>GSAKDPVASAQIELIKQRINNIELFQNNRQAADSALRLEEGILSNAVNSLHRLREIQIQAGNPSLSEEDRKTLAVEAQALLNQLLDYANTKDSNGSYMFSGSKSLTQPVSLNLSGQYVYNGDSTQRFQAVTTSLLVAVNDTGDNVFMRIPSGNGRFAIRETLTPNTGTASVSSGSVTNEAAFVPDNYTMTFALNSQGNLVVMVSGTLSGNVIPPSGLPDDAPLYQEGSAIGFNGMEMVVSGLPKAGDSFSISPAKNESIFSTVQRMINNLNK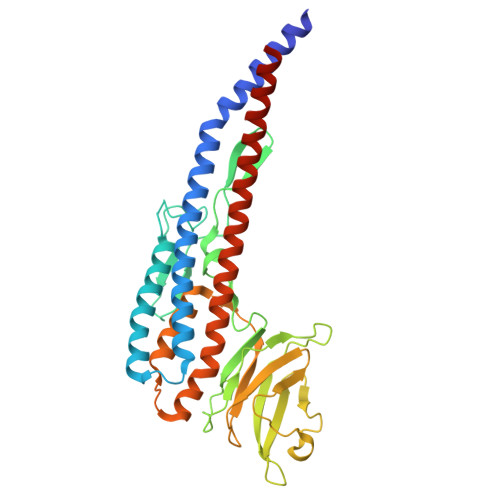PYTSSVEKAATQTENNQLLAQIDSALGHILSVQSDLGARLNQLETAEKANNDYLDISAATLKKLRE[2x]The Redβ protein of the bacteriophage λ red recombination system is a model annealase which catalyzes single-strand annealing homologous DNA recombination. Beta), a 29.7 kDa protein, binds to and protects this exposed nascent ssDNA, catalyzing its annealing to a homologous DNA molecule. λExo and Redβ have been shown to interact in a 1:1 monomer:monomer stoichiometry to form an Exonuclease Annealase Two-component Recombinase (EATR) complex (a.k.a. However, in a manner reminiscent of E. coli SSB, annealases bind to ssDNA, holding it in an extended conformation, removing secondary structures and protecting it from degradation. The N-terminal domain (NTD) mediates oligomerization and contains the catalytic functionality.

We present the structure of the DNA-binding and oligomerization domain of Redβ annealase from phage λ. This structure, resolved to 3.3 Å, was obtained by cryo-EM via helical reconstruction, using a C-terminally truncated Redβ177 bound to two 27mer complementary oligonucleotides. Helical reconstruction and subsequent symmetry determination of the 1-start helical population identified a twist of −12.947 degrees and a rise of 2.078 Å. A single turn of the 1-start helix contains 27.8 asymmetric units, each corresponding to a Redβ177 monomer. In general, the Redβ N-terminal domain consists of a mixed αβ fold consisting of five α-helices, a 310 helix and five β-strands, which form two separate β-sheet elements. The model of Redβ177 was reconstructed as a compact, solenoid, helical filament with dsDNA wound around the outside. This superstructure is stabilized through substantial electrostatic contacts between adjacent monomers in the complex. The outward-facing DNA-binding groove accommodates both strands of the annealed dsDNA product, with an observed stoichiometry of four base pairs per Redβ177 monomer. A total of nine hydrogen bonds between the phosphate backbone and the side chains of R128, W143, H153, K154 and R161 secure the inner, template ssDNA strand in the DNA-binding groove of Redβ177. In addition, the incoming strand is stabilized in a planar orientation through a π-stacking interaction between the phenyl ring of F66 and the purine or pyrimidine ring of the position 3ʹ nucleotide and two hydrogen bonds between R128 and the adjacent nucleotide at position 2ʹ. The annealed duplex DNA is also stabilized in an extended, planar conformation in the DNA-binding groove, which is atypical of B-form helical dsDNA conformations often found in solution. It is likely that upon annealing, the planar conformation is maintained through an induced distortion in the phosphate backbone of the inner (template) DNA strand, which is stabilized by a network of seven hydrogen bonds with R128, W143 and K154.

> MSTALATLAGKLAERVGMDSVDPQELITTLRQTAFKGDASDAQFIALLIVANQYGLNPWTKEIYAFPDKQNGIVPVVGVDGWSRIINENQQFDGMDFEQDNESCTCRIYRKDRNHPICVTEWMDECRREPFKTREGREITGPWQSHPKRMLRHKAMIQCARLAFGFAGIYDKDEAERSSHHHHHH>[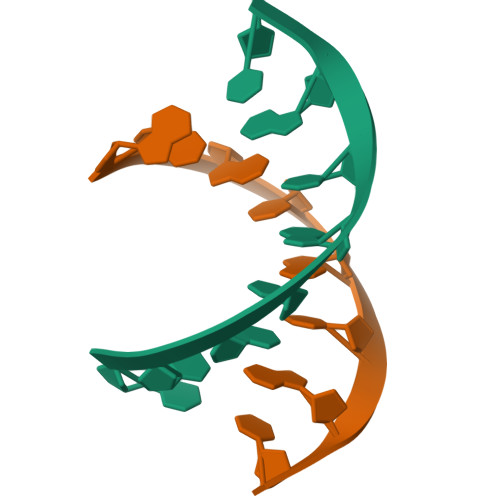2x]GUAUAUAC>GPHMFLKRLDVIGFKSFADRVSIEFVPGVTAVVGPNGSGKSNITDAIRWVLGEQSAKSLRGAKMEDVIFAGSESRKPLNVAEVTITLDNEDGFLPLEYQEVSVTRRVYRSGESEFFINRQPCRLKDIVDLFLDSGLGKEAFSIIGQGRVEEILSSKPEERRTIFEEAAGVLKGSGGGSGEEMKKRFLTTFEQIRAHFGE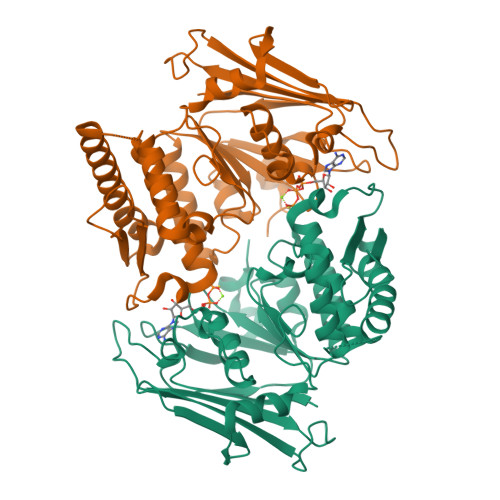VFGELFGGGRADLRLTDPNDLLETGIDIVAQPPGKKLQHLSLLSGGERALTAIALLFSILKVRPVPFCVLDQVEAALDEANVQRYAQYLKRFSRDTQFIVITHRKGTMEEADVLYGVTMQESGVSKLVSVRLEDSKELVRS[2x]> MLKA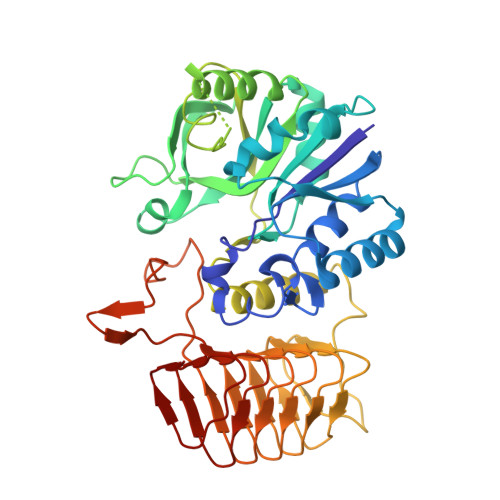VILIGGPQKGTRFRPLSFEVPKPLFPVAGVPMIQHHIEACAQVPGMQEILLIGFYQPDEPLTQFLEAAQQEFNLPVRYLQEFAPLGTGGGLYHFRDQILAGSPEAFFVLNADVCSDFPLSAMLEAHRRQRHPFLLLGTTANRTQSLNYGCIVENPQTHEVLHYVEKPSTFISDIINCGIYLFSPEALKPLRDVFQRNQQDGQLEDSPGLWPGAGTIRLEQDVFSALAGQGQIYVHLTDGIWSQIKSAGSALYASRLYLSRYQDTHPERLAKHTPGGPWIRGNVYIHPTAKVAPSAVLGPNVSIGKGVTVGEGVRLRESIVLHGATLQEHTCVLHSIVGWGSTVGRWARVEGTPSDPNPNDPRARMDSESLFKDGKLLPAITILGCRVRIPAEVLILNSIVLPHKELSRSFTNQIIL>MTGISSKKATIYDLSILSGASASTVSAVLNGSWR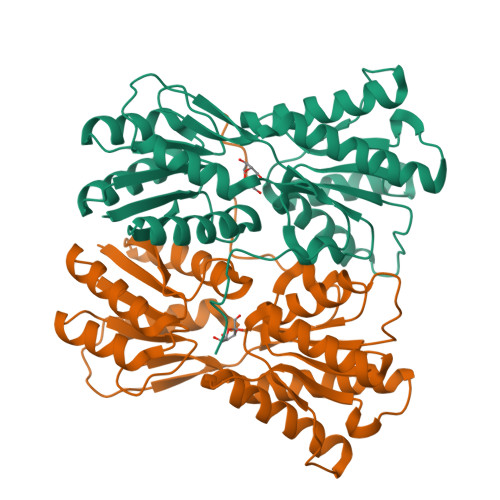KRRISEETADKILSLAKAQRYTTNLQARGLRSSKSGLVGLLVPVYDNRFFSSMAQTFEGQARKRGLSPMVVSGRRDPEEERRTVETLIAYSIDALFIAGVTDPDGVHQVCARAALPHVNIDLPGKFASSVISNNRHGAEILTAAILAHAAKGGSLGPDDVILFGGHDDHASRERIDGFHAAKADYFGVEGGDDIEITGYSPHMTEMAFERFFGRRGRLPRCFFVNSSINFEGLLRFMGRHDGEAFGDIVVGCFDYDPFASFLPFPVYMIKPDIAQMLEKGFELLEENRTEPEVTIIEPQLIPPRTALEGPLDDIWDPVALRRMAK[2x]> MAAQGFLLIATFLLVLMVLARPLGSGLARLINDIPLPGTTGVERVLFRALGVSDREMNWKQYLCAILGLNMLGLAVLFFMLLGQHYLPLNPQQLPGLSWDLALNTAVSFVTNTNWQSYSGETTLSYFSQMAGLTVQNFLSAASGIAVIFALIRAFTRQSMSTLGNAWVDLLRITLWVLVPVALLIALFFIQQGALQNFLPYQAVNTVEGAQQLLPMGPVASQEAIKMLGTNDGGFFN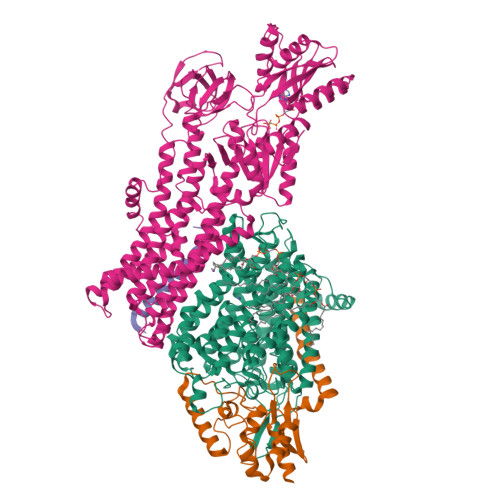ANSSHPFENPTALTNFVQMLAIFLIPTALCFAFGEVMGDRRQGRMLLWAMSVIFVICVGVVMWAEVQGNPHLLALGTDSSINMEGKESRFGVLVSSLFAVVTTAASCGAVIAMHDSFTALGGMVPMWLMQIGEVVFGGVGSGLYGMMLFVLLAVFIAGLMIGRTPEYLGKKIDVREMKLTALAILVTPTLVLMGAALAMMTDAGRSAMLNPGPHGFSEVLYAVSSAANNNGSAFAGLSANSPFWNCLLAFCMFVGRFGVIIPVMAIAGSLVSKKSQAASSGTLPTHGPLFVGLLIGTVLLVGALTFIPALALGPVAEYLS;> MSRKQLALFEPTLVVQALKEAVKKLNPQAQWRNPVMFIVWIGSLLTTCISIAMASGAMPGNALFSAAISGWLWITVLFANFAEALAEGRSKAQANSLKGVKKTAFARKLREPKYGAAADKVPADQLRKGDIVLVEAGDIIPCDGEVIEGGASVDESAITGEAAPVIRESGGDFASVTGGTRILSDWLVIECSVNPGETFLDRMIAMVEGAQRRKTPNEIALTILLIALTIVFLLATATLWPFSAWGGNAVSVTVLVALLVCLIPTTIGGLLSAIGVAGMSRMLGANVIATSGRAVEAAGDVDVLLLDKTGTITLGNRQASEFIPAQGVDEKTLADAAQLASLADETPEGRSIVILAKQRFNLRERDVQSLHATFVPFTAQSRMSGINIDNRMIRKGSVDAIRRHVEANGGHFPTDVDQKVDQVARQGATPLVVVEGSRVLGVIALKDIVKGGIKERFAQLRKMGIKTVMITGDNRLTAAAIAAEAGVDDFLAEATPEAKLALIRQYQAEGRLVAMTGDGTNDAPALAQADVAVAMNSGTQAAKEAGNMVDLDSNPTKLIEVVHIGKQMLMTRGSLTTFSIANDVAKYFAIIPAAFAATYPQLNALNIMCLHSPDSAILSAVIFNALIIVFLIPLALKGVSYKPLTASAMLRRNLWIYGLGGLLVPFIGIKVIDLLLTVCGLV;> MSGLRPALSTFIFLLLITGGVYPLLTTVLGQWWFPWQANGSLIREGDTVRGSALIGQNFTGNGYFHGRPSATAEMPYNPQASGGSNLAVSNPELDKLIAARVAALRAANPDASASVPVELVTASASGLDNNITPQAAAWQIPRVAKARNLSVEQLTQLIAKYSQQPLVKYIGQPVVNIVELNLALDKLDE;> MSAGVITGVLLVFLLLGYLVYALINAE> MENKTETTVRRRRRIILFPVPFQGAINPILQLANVLYSKGFSITIFHTNFNKPKTSNYPHFTFRFILDNDPQDERISNLPTHGPLAGMRIPIINEHGADELRRELELLMLASEEDEEVSCLITDALWYFAQSVADSLNLRRLVLMTSSLFNFHAHVSLPQFDELGYLDPDDKTRLEEQASGFPMLKVKDIKSAYSNWQILKE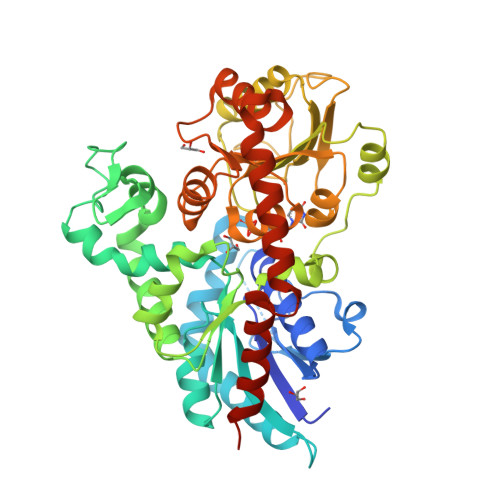ILGKMIKQTKASSGVIWNSFKELEESELETVIREIPAPSFLIPLPKHLTASSSSLLDHDRTVFQWLDQQPPSSVLYVSFGSTSEVDEKDFLEIARGLVDSKQSFLWVVRPGFVKGSTWVEPLPDGFLGERGRIVKWVPQQEVLAHGAIGAFWTHSGWNSTLESVCEGVPMIFSDFGLDQPLNARYMSDVLKVGVYLENGWERGEIANAIRRVMVDEEGEYIRQNARVLKQKADVSLMKGGSSYESLESLVSYISSLLEHHHHHH4-(6-{1-[(R)-S-methanesulfonimidoyl]cyclopropyl}-2-[(3R)-3-methylmorpholin-4-yl]pyrimidin-4-yl)-1H-pyrrolo[2,3-b]pyridine | C20 H24 N6 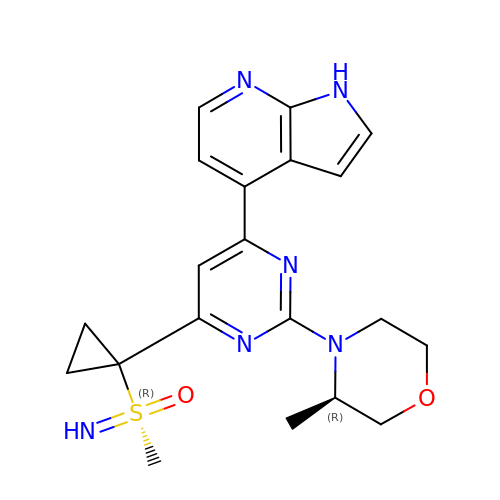O2 S | NQNZWWHMAAZKNQ-JYCIKRDWSA-N> MSKKQEYIAPIKYQNSLPVPQLPPKLLVYPESPETNADSSQLINSLYIKTNVTNLIQQDEDLGMPVDLMKFPGLLN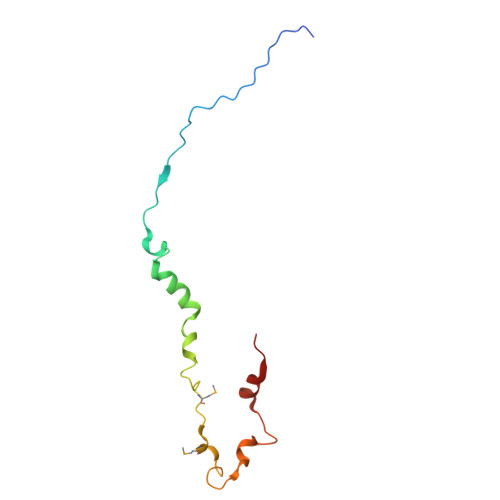KLDSKLLYGFDNVKLDKDDRILLRDPR> MLKQVEIFTDGSCLGNPGPGGYGAILRYRGREKTFSAGYTRTTNNRMELMAAIVALEALKEHCEVILSTDSQYVRQGITQWIHNWKKRGWKTADKKPVKNVDLWQRLDAALGQ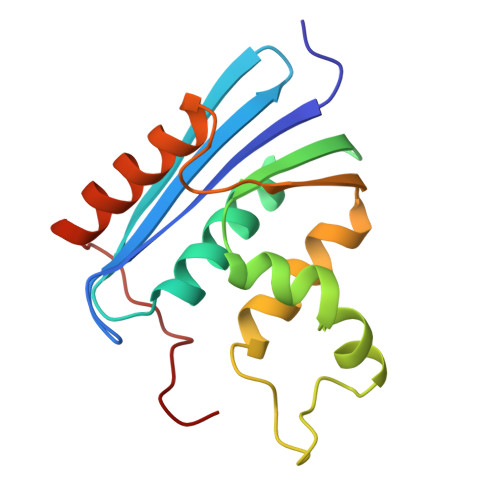HQIKWEWVKGHAGHPENERCAELARAAAMNPTLEDTGYQVEV> MNKQIFVLYFNIFLIFLGIGLVIPVLPVYLKDLGLTGSDLGLLVAAFALSQMIISPFGGTLADKLGKKLIICIGLILFSVSEFMFAVGHNFSVLMLSRVIGGMSAGMVMPGVTGLIADISPSHQKAKNFGYMSAIINSGFILGPGIGGFMAEVSHRMPFYFAGALGILAFIMSIVLIHDPKKSTTSGFQKLEPQLLTKINWKVFITPVILTLVLSFGLSAFETLYSLYTADKVNYSPKDISIAITGGGIFGALFQIYFFDKFMKYFSELTFIAWSLLYSVVVLILLVFANDYWSIMLISFVVFIGFDMIRPAITNYFSNIAGERQGFAGGLNSTFTSMGNFIGPLIAGALFDVHIEAPIYMAIGVSLAGVVIVLIEKQHRAKLKEQNMENLYFQGKLGPEQKLISEEDLNSAVDHHHHHHHHHH;> SVENHWYYFYWYMSP

Efflux pump antiporters confer drug resistance to bacteria by coupling proton import with the expulsion of antibiotics from the cytoplasm. Here, we uncover the proton-coupling mechanism of the Staphylococcus aureus efflux pump NorA by elucidating structures in various protonation states of two essential acidic residues using cryo-EM. NorA contains two essential membrane embedded acidic residues at positions Glu222 and Asp307 which are conserved across S. aureus strains and required for conferring fluoroquinolone resistance to the human pathogen methicillin-resistant S. aureus (MRSA). Hence, the two acidic residues serve as a “belt and suspenders” protection mechanism to prevent simultaneous binding of protons and drug that enforce NorA coupling stoichiometry and confer antibiotic resistance.

Unlike results at pH 7.5, we discovered NorA did not bind to Fab36 at pH 5.0, indicating a unique conformation induced by the lower pH value. We deduced residues Glu222 and Asp307 of NorA were predominantly protonated at pH 5.0 by showing that a double mutant mimicking the protonated state (NorAE222Q,D307N) was unable to bind Fab36 at pH values of 5.0 or 7.5. NorA-FabDA1 and NorAE222Q,D307N-FabDA1 were purified as 1:1 complexes at pH 5.0 and 7.5, respectively, and used for collection of large cryo-EM datasets. Subsequent processing yielded cryo-EM maps at 3.26 Å resolution for NorA and 3.61 Å resolution for NorAE222Q,D307N, which contained the CDRH3 loop or the variable portion of FabDA1 following local refinement. Structures of NorA and NorAE222Q,D307N each displayed the inward-occluded conformation (backbone Cα r.m.s.d of 0.82 Å), where the substrate binding pockets were partially occluded from the cytoplasmic side of the membrane and fully closed from the periplasmic side. For the inward-occluded conformation, TM5 of the NTD was primarily responsible for obstructing the entrance to the substrate binding pocket through interactions with TM7, TM8, TM10, and TM11 of the CTD. Carboxyl groups of Glu222 and Asp307 tethered TM7 and TM10 to TM5 through hydrogen bonds to backbone carbonyls of Phe140 and Ile141 and to the side chain of Asn137, respectively. Nevertheless, the hydrophobicity surrounding these residues likely promotes the occluded conformation by excluding bulk water and reduces the effective dielectric to strengthen the electrostatic interactions involving Glu222 and Asp307. The similarity of interactions with TM5 and overall structural correspondence between wild-type NorA and double mutant structures supported the conclusion that Glu222 and Asp307 were in the protonated forms in the wild-type NorA structure and that the E222Q and D307N mutations suitably mimicked the protonated forms.>MKDLIIPPLDWTQDMGTPKREGAPVHLTIDGVEVTVPAGTSVLRAAAEAGISIPKLCATDNVEPVGSCRLCMVEIEGMRGTPTSCTTPVAPGMRVHTQTPQLQKLRRGVMELYISDHPLDCLTCAANGDCELQDMAGAVGLREVRYQAKDTHFARRDATGPNPRYIPKDNSNPYFSYDPAKCIVCMRCVRACEEVQGTFALTVMGRGFDARISPAAPDFLSSDCVSCGACVQACPTATLVEKSVERIGTPERKVVTTCAYCGVGCSFEAHMLGDQLVRMVPWKGGAANRGHSCVKGRFAYGYATHQDRILKPMIRDKITDPWREVNWTEALDFTATRLRALRDSHGADALGVITSSRCTNEETYLVQKLARAVFGTNNTDTCARVCHSPTGYGLKQTFGTSAGTQDFDSVEETDLALVIGANPTDGHPVFASRLRKRLRAGAKLIVVDPRRIDLLNTPHRGEAWHLQLKPGTNVAVMTAMAHVIVTEQIFDKRFIGDRCDWDEWADYAEFVANPEYAPEAVESLTGVPAGLLRQAARAYAAAPNAAIYYGLGVTEHSQGSTTVIAIANLAMMTGNIGRPGV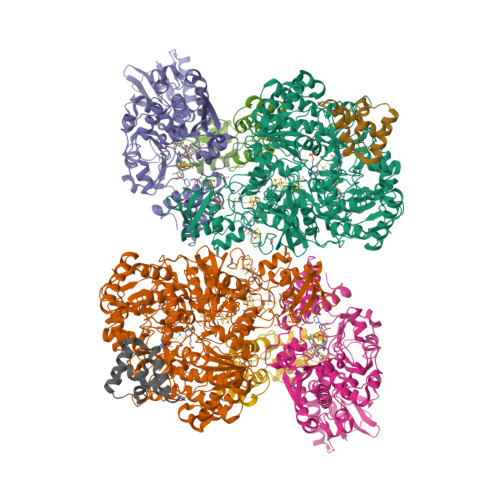GVNPLRGQNNVQGSCDMGSFPHEFPGYRHVSDDATRGLFERTWGVTLSSEPGLRIPNMLDAAVEGRFKALYVQGEDILQSDPDTRHVSAGLAAMDLVIVHDLFLNETANYAHVFLPGSTFLEKDGTFTNAERRINRVRRVMAPKAGFADWEVTQMLANALGAGWHYTHPSEIMAEIAATTPGFAAVTYEMLDARGSVQWPCNEKAPEGSPIMHVEGFVRGKGRFIRTAYLPTDEKTGPRFPLLLTTGRILSQYNVGAQTRRTENTVWHGEDRLEIHPTDAETRGIRDGDWVRLASRAGETTLRATVTDRVSPGVVYTTFHHPDTQANVVTTDTSDWATNCPEYKVTAVQVAASNGPSDWQQDYAAQAAAARRIEAAE[2x];>[2x]MKIWLPCDAAAKACGAEAVLAALRLEAEKRGGALDIARNGSRGMIWLEPLLEVETPAGRIGFGPMTPADVPALFDALESHPKALGLVEEIPFFKRQTRLTFARCGRIEPLSLAQFAAAEGWAGLRKALKMTPAEVVEEVLASGLRGRGGAGFPTGIKWRTVAAAQADQKYIVCNVDEGDSGSFADRMLIEGDPFCLVEGMAIAGHAVGATRGYVYIRSEYPDAIAVMRAAIAMAKPFLAEAGFEMEVRVGAGAYVCGEETSLLNSLEGKRGTVRAKPPLPALKGLFGKPTVVNNLLSLAAVPWIIAHGAKAYESFGMDRSRGTIPLQIGGNVKRGGLFETGFGITLGELVEDICGGTASGRPVKAVQVGGPLGAYHPVSDYHLPFCYEQFAGQGGLVGHAGLVVHDDTADMLKLARFAMEFCAIESCGTCTPCRIGAVRGVEVIDRIAAGDASAMPLLDDLCQTMKLGSLCALGGFTPYPVQSAIRHFPADFPCAREAAE;>[2x]MTDTARLRAILAAHRGREGALLPILHDVQAAFGFIPEDAYAPIAADLGLTRAEVAGVVGFYHDFRKAPAGRHVIKLCRAEACQAMGMDAVQARLESALGLRLGDSSEAVTLEAVYCLGLCACAPAAMVDDRLVGRLDAAAVAGIVAELGA;>MSDDKIIRMANQIAAFFAVQPGDRAGPVAAHISENWSAPMRAALLAHVAAQSPGLDPLVIAAAPQIRPVPA[2x]>[2x]MATFYEVIVRVPFDVEEHLPGISDSFVDWVTGQIWELPPESDLNLTLVEQPQLTVADRIRRVFLYEWNKFSKQESKFFVQFEKGSEYFHLHTLVETSGISSMVLG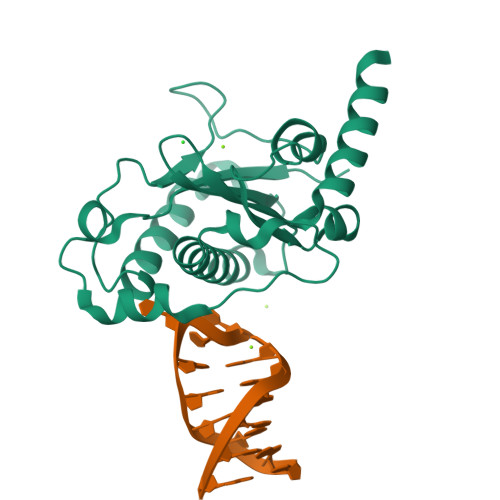RYVSQIRAQLVKVVFQGIEPQINDWVAITKVKKGGANKVVDSGYIPAYLLPKVQPELQWAWTNLDEYKLAALNLEERKRLVAQFLAESSQRS> GAMGGWAIAVHGGAGVDPTLPLERQEEAKQLLTRCLNLGISALNSNVPAIDVVELVVRELETDPLFNSGRGSALTEKGTVEMEASIMDGPKRRCGAVSGLTTVKNPISLARLVMDKSPHSYIAFSG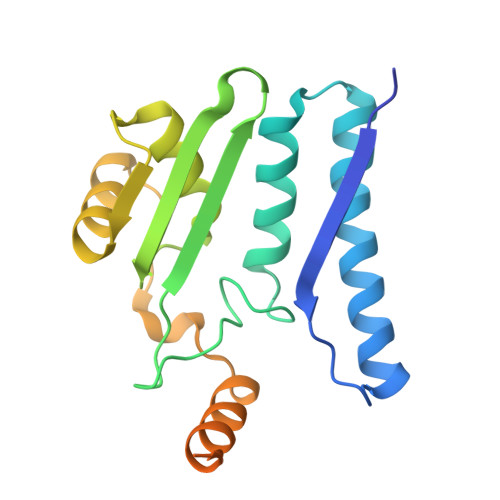AEDFARQQGVEVVDNEYFVTPDNVGMLKLAKEANTILFDYRIPSSAYETCGSGVESPLQMNGLPISVYAPE4-{[5-({(2S)-2-butyl-5-oxo-4-[3-(trifluoromethoxy)phenyl]piperazin-1-yl}methyl)-1H-imidazol-1-yl]methyl}-2-fluorobenzonitrile 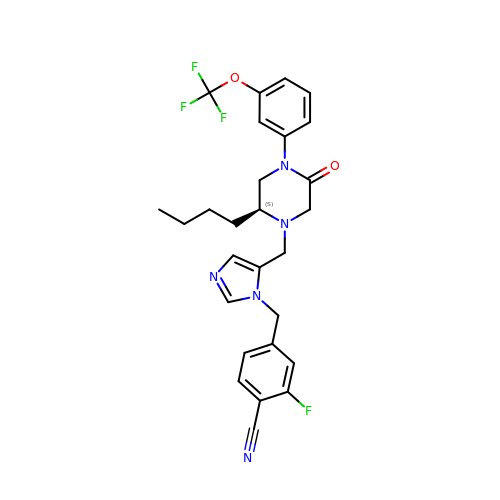| C27 H27 F4 N5 O2 | WRNSPFWIUHUJNC-QFIPXVFZSA-N> METIGNFIQNMAFPTENPYKLSGDFGNSTLEPTVTAALRILHESPAPFNTEFFSRKNVDF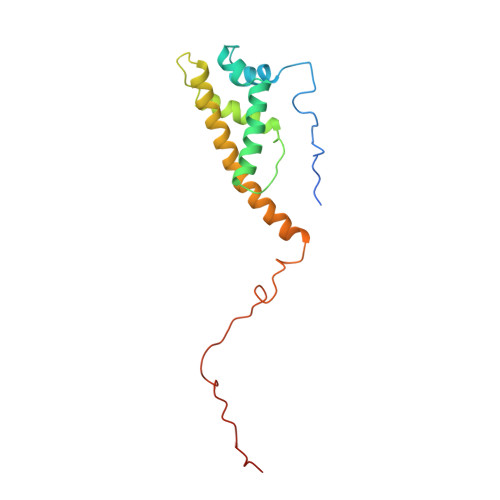IQKKLISETKRYTSFDIGPQNEDELIMMMAGIYVQDSTFDGNIKAGLRKLNTLVITECLKQILPGVRAYALYVRDASLPFSGGGEEAFKRPELATLKGSKVLSGFLPLDRNAS>MRGLSRRVQAMKPSATVAVNAKALELRRQGVDLVALTAGEPDFDTPEHVKEAARRALAQGKTKYAPPAGIPELREALAEKFRRENGLSVTPEETIVTVGGKQALFNLFQAI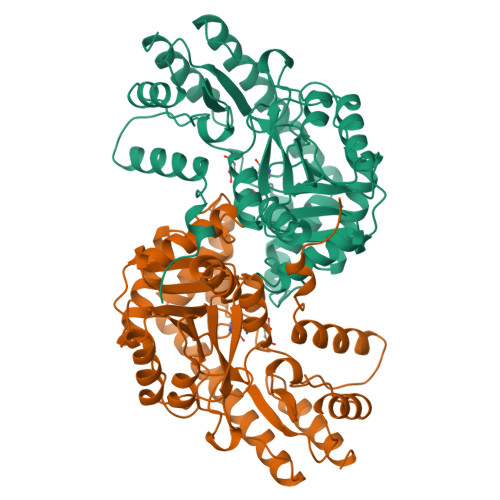LDPGDEVIVLSPYWVSYPEMVRFAGGVVVEVETLPEEGFVPDPERVRRAITPRTKALVVNSPNNPTGAVYPKEVLEALARLAVEHDFYLVSDEIYEHLLYEGEHFSPGRVAPEHTLTVNGAAKAFAMTGWRIGYACGPKEVIKAMASVSSQSTTSPDTIAQWATLEALTNQEASRAFVEMAREAYRRRRDLLLEGLTALGLKAVRPSGAFYVLMDTSPIAPDEVRAAERLLEAGVAVVPGTDFAAFGHVRLSYATSEENLRKALERFARVLGRA[4x]> MGAWAMLYGVS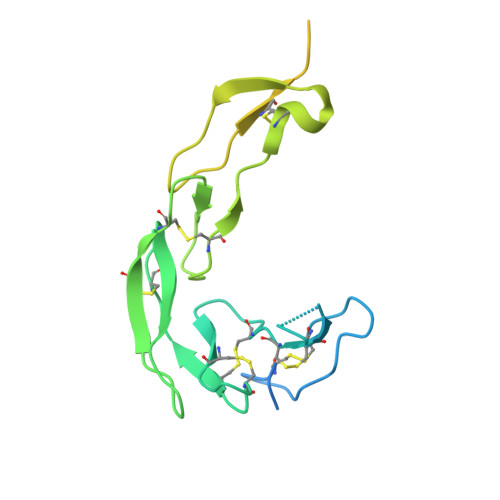MLCVLDLGQPSVVEEPGCGPGKVQNGSGNNTRCCSLYAPGKEDCPKERCICVTPEYHCGDPQCKICKHYPCQPGQRVESQGDIVFGFRCVACAMGTFSAGRDGHCRLWTNCSQFGFLTMFPGNKTHNAVCIPEPLPTEQYGHLTVIFLVMAACIFFLTTVQLGLHIWQLRRQHMCPRETQPFAEVQLSAEDACSFQFPEEERGEQTEEKCHLGGRWP>[4x]MGTKKSAAEASKKPRQKRTAT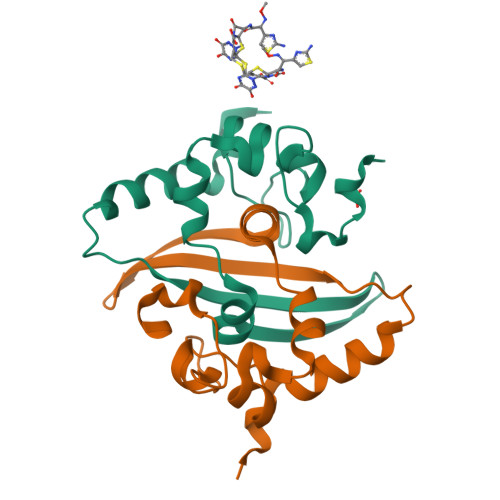KAYNVTQAFGRRGPEQTQGNFGDQELIRQGTDYKHWPQIAQFAPSASAFFGMSRIGMEVTPSGTWLTYTGAIKLDDKDPNFKDQVILLNKHIDAYKTFPPTEPKKDKKKKADETQALPQRQKKQQTVTLLPAADLDDFSKQLQQSMSSADSTQA> SNAMRIGHGFDVHKFGENGSG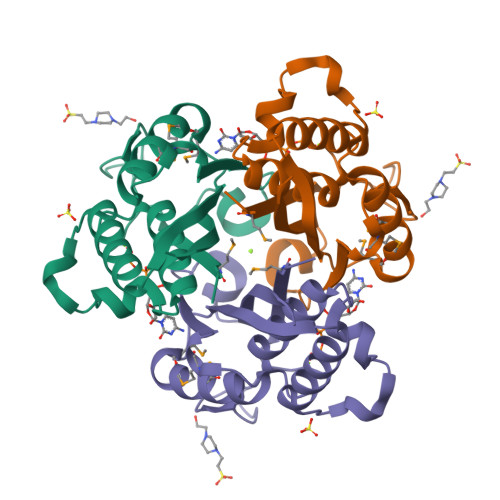PLIIGGVRIPYEKGLLAHSDGDVALHAATDALLGAAALGDIGKLFPDTDPAFKGADSRGLLREAYRRILAKGYKLGNLDITIIAQAPKMAPHIPQMRVNLAEDLQCHMDDINVKATTTEQLGFTGRGEGIACEAVVLLVNVEQG> EVFKGHNLPRLRGAMIGPHVTNADLLEFGNVWKANHIRWQLIWNGFPHSPADSATLDEYRQWLDGALKRLEAALPVCREAGILVTVDLHTPPGGRNEASECRIFHDREFQKAFIDIWEDIARRFADSDVVWGYDLVNEPVE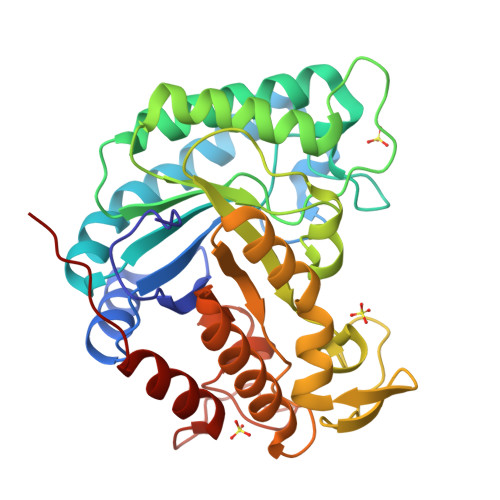GMVPDGLMNWQRLAEETARRVRAIDQKHAIIIEPAPWGSPSSIALLDPIDVPGVVYSVHMYVPHAFTHQGVYDNPVGIVYPGTIDGKWYDRNTLRKVLEPVRRFQEENGVHIYIGEFSAIRWAPADSACQYLKDCIEIFEEYGWDWAYHAFREWDGWSVEHGPDRNDRNRTATPTDRALLLRSWYAENVKPQFS> DSSTTKDVIQKGISVVGDLLGVVGFPFGGALVSFYTNFLNTIWPSEDPWKAFMEQVEALMDQKIADYAKNKALAELQGLQNNVEDYVSALSSWQKNPVSSRNPHSQGRIRELFSQAESHFRNSMPSFAISGYEVLFLTTYAQAANTHLFLLKDAQIYGEEWGYEKEDIAEFYKRQLKLTQEYTDHCVKWYNVGLDKLRGSSYESWVNFNRYRREMTLTVLDLIALFPLYDVRLYPKEVKTELTRDVLTDPIVGV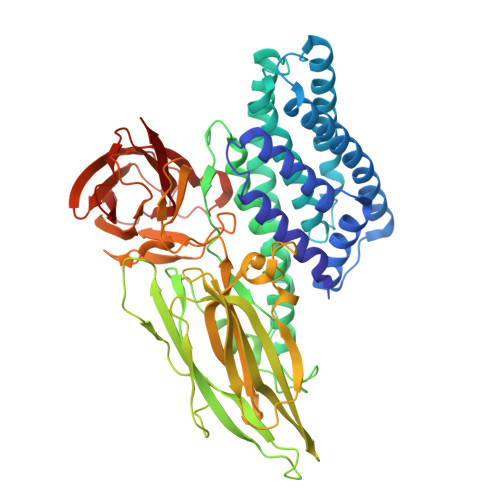NNLRGYGTTFSNIENYIRKPHLFDYLHRIQFHTRFQPGYYGNDSFNYWSGNYVSTRPSIGSNDIITSPFYGNKSSEPVQNLEFNGEKVYRAVANTNLAVWPSAVYSGVTKVEFSQYNDQTDEASTQTYDSKRNVGAVSWDSIDQLPPETTDEPLEKGYSHQLNYVMCFLMQGSRGTIPVLTWTHKSVDFFNMIDSKKITQLPLVKAYKLQSGASVVAGPRFTGGDIIQCTENGSAATIYVTPDVSYSQKYRARIHYASTSQITFTLSLDGAPFNQYYFDKTINKGDTLTYNSFNLASFSTPFELSGNNLQIGVTGLSAGDKVYIDKIEFIPVN>GPGSESSNISQESKLINTLTDENEKLREELQQYYALSDAKEEEPRYKALRGENQDLREKERKYQDKIKKLEEKEKNLEKKSED[4x];>GPGSNCGPPPTLSFAAPMDITLTETRFKTGTTLKYTCLPGYVRSHSTQTLTCNSDGEWVYNTFCIYKRCRHPGELRNGQVEIKTDLSFGSQIEFSCSEGFFLIGSTTSRCEVQDRGVGWSHPLPQ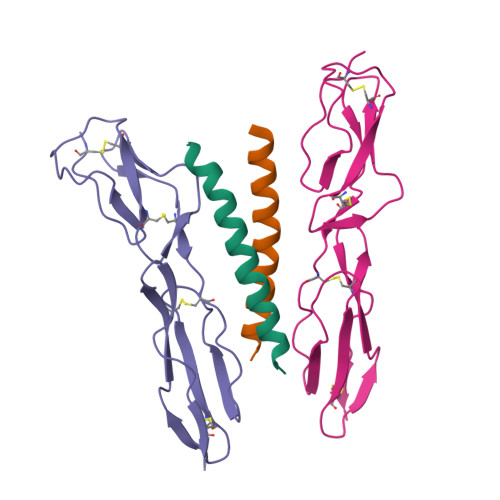CEI[4x]>GADIDKNAKLQTTVKVNEQVSTTTKSVEVPENKDGVKVVDTLHYKGLVAGEKYEVKGTIYAVNGDNEEEVKE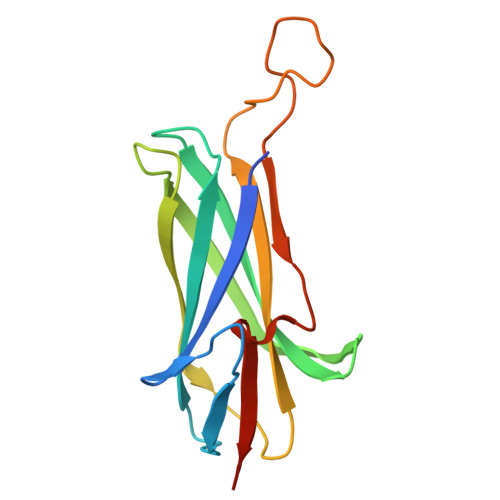TKTAEFTADASGQGDWDLDFGSVKNLEAGKSYVVYEEVTSKENLVDKDNNGTPDEKQTLEHKDPKDKAQIMVIKPKTEKE[2x]> EEVLLDTTGETSEIGWLTYPPGGWDEVSVLDDQRRLTRTFEACHVAGAPPGTGQDNWLQTHFVERRGAQRAHIRLHFSVRACSSLGVSGGTCRETFTLYYRQAEEPDSPDSVSSWHLKRWTKVDTIAADESFPSSSSSSSSSSSSAAWAVGPHGAGQRAGLQLNVKERSFGPLTQRGFYVAFQDTGACLALVAVRLFSYTCPAVLRSFASFPETQASGAGGASLVAAVGTCVAHAEPEEDGVGGQAGGSPPRLHCNGEGKWMVAVGGCRCQPGYQPARGDKACQACPRGLYKASAGNAPCSPCPARSHAPNPAAPVCPCLEGFYRASSDPPEAPCTGPPSAPQELWFEVQGSALMLHWRLPRELGGRGDLLFNVVCKECEGRQEPASGGGGTCHRCRDEVHFDPRQRGLTESRVLVGGLRAHVPYILEVQAVNGVSELSPDPPQAAAINVSTSHEVPSAVPVVHQVSRASNSITVSWPQPDQTNGNILDYQLRYYDQAEDESHSFTLTSETNTATVTQLSPGHIYGFQVRARTAAGHGPYGGKVYFQ

Eph receptors are the largest group amongst the receptor tyrosine kinases and are divided into two subgroups, A and B, based on ligand binding specificities and sequence conservation. The extracellular region of Eph receptors includes an N-terminal ligand-binding domain, followed by a cysteine-rich region and two fibronectin-type-3 domains. Generally Eph receptor signaling relies on their kinase activity, but both EphA and EphB classes contain innately kinase-deficient members, EpA10 and EphB6, that lack catalytic activity because of alterations of conserved motifs within their kinase domains. Due to the absence of the intrinsic kinase activity, EphB6 often operates by interacting with kinase-active Eph receptors and these interactions likely determine the signaling outcomes in varying biological contexts.

The C-terminal FN3 domain is not clearly visible in the electron density map, similar to the EphA2-ECD crystal structure, consistent with its increased flexibility in relation to the rest of the Eph ectodomain. First, inside the LBD, EphB6 has an insert of 11 consecutive Serine residues within the J-K loop (residues 151–161 in our construct). Indeed, this highly flexible serine insert might interfere with ligand binding by hindering the formation of a well-defined ligand-binding cavity on the receptor surface. Second, the H-I loop, N-terminal to the J-K loop (residues 125–130 in our structure) represents another unique to EphB6 Serine-rich motif, which is fully structured. Finally, the first FN domain of EphB6 has a seven-residue insertion in the loop between E-396 and G-406 and hence, adopts a significantly different conformation than the one observed in EphA2 or EphA4. We suggest, though, that because EphB6 is kinase inactive and obligated to use other Ephs as co-receptors to effect signaling, this loop might be part of an Eph-Eph oligomerization interface, to mediate interactions between EphB6 and other receptors (e.g. EphA2) within the same Eph/ephrin signaling assemblies. Our structural analysis shows that, similar to the A-class Eph-ECD structures published earlier, the ectodomain of the unliganded EphB6 receptor also participates in LBD-FN3 head-to-tail interactions with its neighboring molecules. The total buried area of this interface is 860 Å, close to that for EphA2 (980 Å) (unpublished data) but much smaller than the one reported for EphA4 (2,460 Å).> MEAGYAEIAAVQFNIAGDNDHKRQGVMEVTISNLFEGTLPAEGGIYDARMGTTDHHYKCITCSHQRKQCMGHPGILQMHAPVLQPLFIAEIRRWLRVICLNCGAPIVDLKRYEHLIRPKRLIEAASSQTEGKQCYVCKAVHPKIVKDSEDYFTFWVDQQGKIDKLYPQIIREIFSRVTYDTVVKLGRSKNSHPEKLVLKAIQIPPISIRPGIRLGIGSGPQSFHDINNVIQYLVRKNLLIPKDLQIVRGQKIPLNIDRNLQTIQQLYYNFLLDSVSTTATQGGTGKRGIVMGARPAPSIMRRLPRKEGRIRKSLLGSQVWSISRSTICGNSDLHLDEVGYPISFARTLQVAETVQHYNINRLMPYFLNGKRQYPGCSRVYKQITQSVHDIEGLKQDFRLEVGDILYRDVVTGDVAFFNRQPSLERSSIGVHRIVVLENPKISTFQMNVSACAWYNADFDGDQMNLWVPWSVMSRVEAELLCSVRNWFISTKSSGPVNGQVQDSTVGSFLLTRTNTPMGKNVMNKLHAMGLFQTTQTDPPCFANYSPTDLLDGKSVVSMLLKQTPINYQRAPTWYSEVYAPYMHYNKQDISTQIRNGELIEGVLDKKAVGAGSSGGIYHLISRRYGPQQALKMIFATQQLALNYVRNAGFTVSTADMLLTPEAHQEVQEIINKLLLESEEINNRLLHGDIMPPIGLTTHDFYEKLQLNALKFPDRILKPIMNSINPETNGLFQMVATGAKGSNPNMIHIMAGIGQIEINTQRIQPQFSFGRTLVYYPRFALEAQAYGFICNSYIAGLTSPEFIFGEMNGRFDLINKALSTSSTGYANRKAIFGLQSCIVDYYRRVSIDTRLVQQLYGEDGLDARQLETVRFETIMLSDQELEDKFKYTGIQSPLFEEEFSRLKKDRDKYRQIFLNVENFNFSQLLTDVRQVPVNVASIVKNILLSSTSGVLPFDEKSILQKYAMVKTFCKNLPYVFINNIQERLQTPIPVYLKRAAALMRMLIRIELATVKTLNITCEQMSAILDLIRLQYTQSLINYGEAVGILAAQSVSEPLTQYMLDSHHRSVAGGTNKSGIVRPQEIFSAKPVEAEQSSEMLLRLKNPEVETNKTYAQEIANSIELITFERLILQWHLLYETYSSTKKNVMYPDFASDVEWMTDFLENHPLLQPPEDIANWCIRLELNKTTMILKSISLESIINSLRAKHPNTYIMHSVENTASGIPIIIRIYLRESAFRRSTNTRMATDEKIAVNVVDKLLNSTIRGIPGIKNANVVKLMRHRVDAQGKLVRLDNIYAIKTNGTNIFGAMLDDNIDPYTIVSSSIGDTMELYGIEAARQKIISEIRTVMGDKGPNHRHLLMYADLMTRTGQVTSLEKAGLNAREPSNVLLRMALSSPVQVLTDAAVDSAVNPIYGIAAPTLMGSVPRIGTMYSDIIMDEKYITENYKSVDSMIDML;> GMEPLRPQITYGPIETVDNEELTEADMLSFISAAVNSTGLIGYNIKSFDDLMDNGIPQIVKQMFNVDITYKDQRDHTEIDKLRESVQIQFNFTDVNIERPQHRNYSQGNKINLLPNKARLCGLSYSGPVNLAAEVILTAHYSNGRQEVKRASIPPFQVSTFPIMRGSNRCHTHHLSKTAKKEIGEDPNEPGGYFIARGGEWVVDLLENIRFNTLHIHYHTMQQGNNEIIRGEFISQPGGAFENSSQIIIRYMTTGAITIEINSTKFSKLRIPWYLIFRMFGMTGDDSIIEQVVFDLESNSPVNTFMIEILEKSIHVLDPIFQPVQHEPNREKIIQFLSEKVSKFVSNPSAYKSDENAVQYLNERQLTILDKILLPHMGQTADTRVRKLRFLGLLIHKILLVIMNVFPPTDRDSYRTKRVHGSGVSLAKAFKAIFNTSVIAPIINGFKELLKQTAFEELTQRNIIEAFSAALSKNTASDLNRSMEQSIISGNKTIMVRQRPIVNRVSTQSLERKNLLNTISALRTVNTHNTTNASKQTERADMMRRVHASYPGYICVAQSADTGEKVGMSKQLAITANVCTAGEVLSLKQRLLSDPAIQQLADVSNKDIVRKGLARVFINGEWIGCCTNAFELAQRYRMFRREGKIVHPHTTIYWDSMVDEVEFWLDVGRLTRPLLIVDNNIEKYNQACYKAAEARKKGDKDWEKHKIPFIQNTRFTSQMAKDILAGTLTLEDLVAQGICEFITPEEAENCLVAFSIIELRKHKHDVTRRFTHVDVPQAILGLAALVSPYANCTQPARVTYETNQGRQTGGWYCFSWPYRVDMNRFFQFYNEMPLVKTIAHNYVIPNGLNTIVAYMIYGGYNQEDSVIVSQSFIDRGGFAGTFYREEKVELESDIESFGKPDPLITKNLKPGANYEKLVDGFVPVGTVVKKGDIIIGKVAKIRGEKDELNKYIDRSVMYGFDEPAVVDAVMRPHGPNDEIFGLMRLRYERNLNIGDKMSSRSGNKGIAALALPTSDMPFTEDGLQPDLIVNPHSHPSRMTNGQMIETTVGLANALQGVVTDGTAFLPINVQLLSERLAQEGLRFNGCQKMFNGQTGEYFDAAIFIGPTYHQRLQKFVLDDRYAVASYGPTDALTGQPLDGKRSHGGLRLGEMEHWVLTAQGAMQTIIEKSHDDSDGCISYICRNCGEPAIYNASHPIYKCMNCDVQADIGMVDSRRSSIVFQHEMRAANVNITSVLSPRVFQPA;> MEKIFQNVEIKPFLIDFSNPFIKNAAKRLFQLEEQLPLVPVNVVMDFKGISRAAVHGLSRVLQDEIPNYMLDIKPGGYKIEDSTDLFMTEQFIRNRINFIPIYAKNETLVFALRSLNNSCEVKTIYSRDLIQVAGPKLKYPIFNPTFEIGFLQPGKSLIIEDIYIKKGIGRKHAAFNLAVKTHFSHLDIEQYPTDKKEYMALSGYKQSSMTSDPRHHRLGLCFPAVPLPHINQAVRTYLKNACRIIIGRIQSIQKIYENFEEPQPELVLFSLDEEKTKAIITIKDETHTIGNLLKTCIYEMIPDISFVGYQCVPHKQEMVLTIIHKASQEDLITLLEKSIQNIIQTFQILEKNVDELIA;> MIDQKIFETTLNIDDPTNFCTNVEAHLLKELENIYVGKCFKNSFILNITGVIQRSPCFIMRTNNSGRGYMHVRFSAVVSYLNAFDLIAAVKIIKNDSNIILGESLLTEPVTIVIPSSESQNNVAEVGQIVPVQLANSSVYYIPGRQQASATGSIFIPKHTFSVYHVQEELTQEQALNLTKLVNIIEMLLESRSKKDFKQICFFEKLYYTYSISSDEILDLKIWKGPKGKEMSRLKPCNVLSFLYDALKNKSSSLGFWARPPNLLKSSPLAYQQDQNSFNATELPIICSAEVMFVTLLKEIINYLQFMNDLCDTFNNEQLIKRHENIWMLIEQRKIGHDF;> MAMQKLFTYIYEFIEYRKMVLLEEKVPYDKFVQMVLNTGFFRINAETLNHGIVSVFIFGANGKYVHHGGDMRTLLTNTLNEKKHYEELILIVDKPVLSKKNILDIIVEQRAANPTIVINIYPYHLFCINIPKVSAIPKHKLITQEEAQEFLGREYLQPQDLMQISASDPPVVWLGGRPGDFVQIERPSETAMHAVVIRFITKSKI;> MADNDNEDIIMDDLVEEYVETEEENFVDSEEESEDKDEIVESPSICEGFVQASSQTLVIIPDNERITSNVLTTFEATRLVAVRAQQLAINGSTMLKKKYSSPIDIAKQELFNRKIPLLVMRCIKVTPEGQKIVEIWNPREMGIPLLD;> MKICKACSSCMVRTYVDGNIIFRCSCGESVQGDSQNLLVSSKVYHTGEMEDKYKIFIKNAPFDPTNCQIKKDCPNCHLDYLTQICIGSQKIIILVCRCGYMSNRG;> MLIPVVCFTCGFPIGTYAAIFDKARTEYIKTKMDGTLPQNIPLDASLQIELKDLITALGIPMRVCCRTHLITTLDYRKYY

African Swine Fever Virus is a Nucleo-Cytoplasmic Large DNA Virus that causes an incurable haemorrhagic fever in pigs with a high impact on global food security. ASFV replicates in the cytoplasm of the infected cell and encodes its own transcription machinery that is independent of cellular factors, however, not much is known about how this system works at a molecular level. The ASFV RNAP bears a striking resemblance to RNAPII with bona fide homologues of nine of its twelve subunits. Key differences include the fusion of the ASFV assembly platform subunits RPB3 and RPB11, and an unusual C-terminal domain of the stalk subunit vRPB7 that is related to the eukaryotic mRNA cap 2´-O-methyltransferase 1.

We have solved the cryo-EM structures of the RNAP with the clamp in closed and open conformations at 2.7 and 2.9 Å resolution, respectively. We solved the structure of the ASFV core RNAP in two conformations, i. e. an open and closed state, which refer to the mobile RNAP clamp and the width of the DNA-binding channel. Subsequently, the batches of corresponding particles were isolated and provided two maps at the nominal resolution of 2.73 Å for the closed conformation, and 2.92 Å for the open conformation. However, to achieve better structural information for the protrusion and wall domains, we employed a new refinement method, named 3DFlex refinement, applied after 3D refinement of the closed conformation map. The new refinement produced a higher quality map, improving the local resolution in particular of mobile domains exposed on the surface like vRPB5, vRPB7, whose map quality was comparable to the multibody refinement result, and the protrusion (for comparison see Supplementary Figs. 3a and 4a). The active centre is well resolved in both the closed and the open RNAP conformation maps showing the catalytic magnesium A ion (Mg A) fully coordinated by the aspartate triad D457, D459, and D461 in the conserved NADFDGD motif. The bridge helix (BH) is in the straight conformation, while the trigger loop (TL) is structurally well-defined in both closed and the open ASFV RNAP structures. We identified two additional densities of unknown nature in both maps of the closed and the open RNAP. The first density is located inside the DNA-binding channel, forming a stacking interaction with the side chain of residue Y824 on the bridge helix (BH) and surrounded by several positively charged residues. The second density is located at the foot domain of vRPB1, and also surrounded by positively charged residues.> MAAAVAMETDDAGNRLRFQLELEFVQCLANPNYLNFLAQRGYFKDKAFVNYLKYLLYWKDPEYAKYLKYPQCLHMLELLQYEHFRKELVNAQCAKFIDEQQILHWQHYSRKRM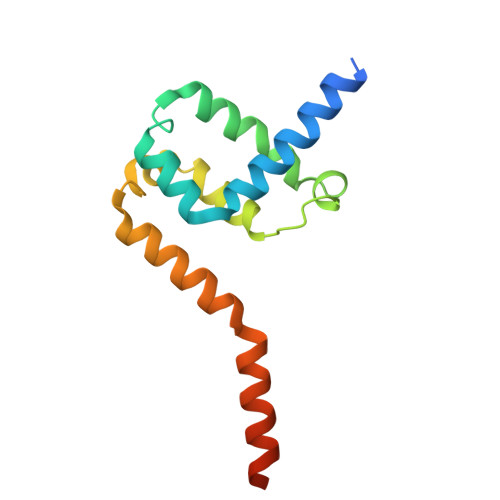RLQQALAEQQQQNNTSGK> GSSTPLVDFLMQLEDYTPTIPDAVTGYYLNRAGFEASDPRIIRLISLAAQKFISDIANDALQHCKMKGTASGSSRSKSKDRKYTLTMEDLTPALSEYGINVK;> MPADNYHLARRRTLQVVVSSLLTEAGFESAEKASVE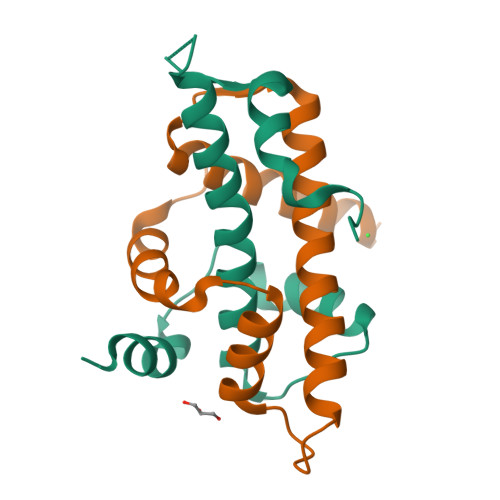TLTEMLQSYISEIGRSAKSYCEHTARTQPTLSDIVVTLVEMGFNVDTLPAYAKRSQRMVIT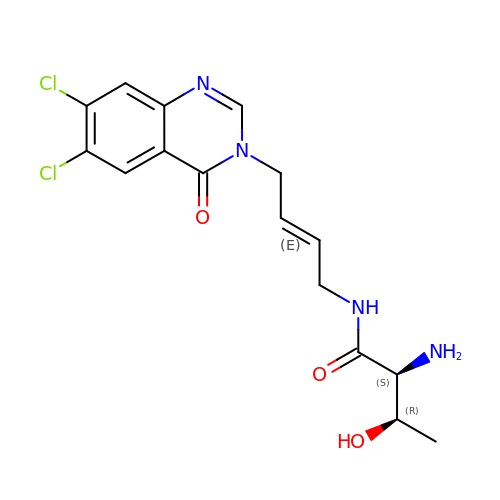(2S,3R)-2-azanyl-N-[(E)-4-[6,7-bis(chloranyl)-4-oxidanylidene-quinazolin-3-yl]but-2-enyl]-3-oxidanyl-butanamide | C16 H18 Cl2 N4 O3 | YXMAQAPNMNRQQB-XKKUMHBKSA-N> HHHSSGLVPRGSHMANKAVNDFILAMNYDKKKLLTHQGESIENRFIKEGNQLPDEFVVIERKKRSLSTNTSDISVTATNDSRLYPGALLVVDETLLENNPTLLAVDRAPMTYSIDLPGLASSDSFLQVEDPSNSSVRGAVNDLLAKWHQDYGQVNNVPARMQYEKITAHSMEQLKVKFGSDFEKTGNSLDIDFNSVHSGEKQIQIVNFKQIYYTVSVDAVKNPGDVFQDTVTVEDLKQRGISAERPLVYISSVAYGRQVYLKLETTSKSDEVEAAFEALIKGVKVAPQTEWKQILDNTEVKAVILGGDPSSGARVVTGKVDMVEDLIQEGSRFTADHPGLPISYTTSFLRDNVVATFQNSTDYVETKVTAYRNGDLLLDHSGAYVAQYY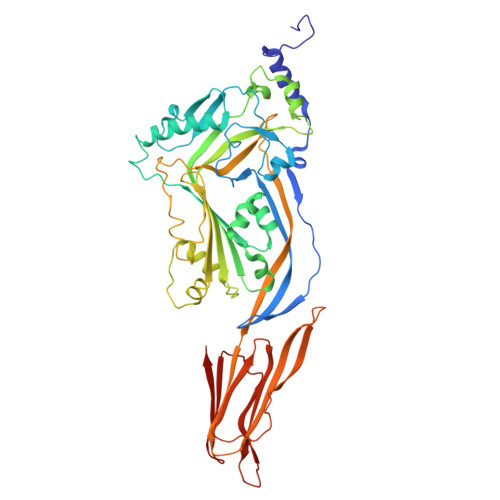ITWNELSYDHQGKEVLTPKAWDRNGQDLTAHFTTSIPLKGNVRNLSVKIRECTGLAWEWWRTVYEKTDLPLVRKRTISIWGTTLYPQVEDKVEND> MACPSQCSCSGTTVDCSGKSLASVPTGIPTTTQVLYLYDNQITKLEPGVFDRLTQLTRLDLDNNQLTVLPAGVFDKLTQLTQLSLNDN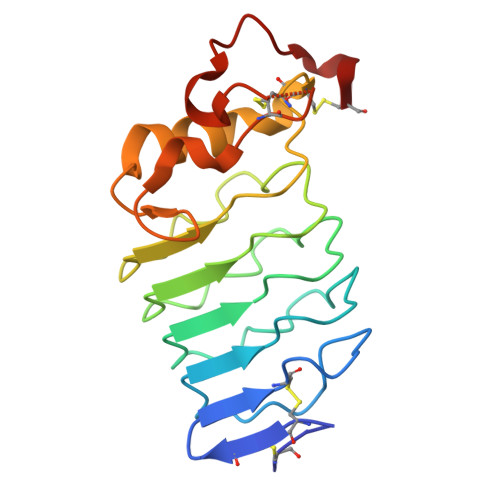QLKSIPRGAFDNLKSLTHIWLLNNPWDCACSDILYLSRWISQHPGLVFGYLNLDPDSARCSGTNTPVRAVTEASTSPSKCPG The Carboxyl terminus of the HSC70 interacting protein (CHIP) is an E3 ligase that blocks the ATPase activity of HSP(C)70 and tags substrates with ubiquitin for degradation. CHIP has three functional domains: a tetratricopeptide (TPR) domain for binding to chaperones, a coiled-coil domain, and a U-box domain where ubiquitin binds before transfer to a substrate. The opposing co-chaperone to CHIP is HSP organizing protein (HOP), which also contains multiple TPR domains and increases HSP(C)70’s ATP hydrolysis, enhancing substrate refolding. Both co-chaperones interact via the EEVD motif in the C-terminal tail of HSP(C)70, making this domain a significant mechanism in chaperone function and a therapeutic target. To understand the structural interactions of HSP70 and CHIP at the atomic level, we completed structural studies of the CHIP-TPR domain of CHIP (21–154) with either the phosphorylated or unmodified tail of HSP70.

Although the new structures of CHIP-TPR with HSP70 peptide and pT-HSP70 peptide are globally similar and nearly identical, key differences are observed for T636 and neighboring HSP70 peptide residues. First, the position of the HSP70 tail near T636 is different across the structures, indicating the potential flexibility of this region, the potential for this region to adopt more than one conformation, or the presence of crystal contacts forcing one conformation or the other in various crystal packing arrangements. Second, the position of the T636 side chain in the CHIP-TPR HSP70 peptide complex is not available to pThr636 in the CHIP-TPR pT-HSP70 peptide complex because this would place the phosphate group of pT636 in close proximity to D134 of the CHIP-TPR. If this mutation is made in CHIP with non-phosphorylated HSP70, there is no contact between N132 and HSP70, so modeling predicts that G132N should not affect non-phosphorylated HSP70. Due to the position of the N132 side chain, removing the pT636 phosphate group would not result in any steric clashes; therefore, the EEVD tail structure could return to that seen in the CHIP-TPR/HSP70-SBD or CHIP-TPR/HSP70 peptide structures.

> GAMGSEKSPSAQELKEQGNRLFVGRKYPEAAACYGRAITRNPLVAVYYTNRALCYLKMQQHEQALADCRRALELDGQSVKAHFFLGQCQLEMESYDEAIANLQRAYSLAKEQRLNFGDDIPSALRIAKKKRWNSIEERR;> GPTIEEVD>[4x]AMAISDPQAENPIFTDVFTADPAALVHKGRVYLYAGRDEAPDNTTFFVMNEWLVYSSDDMANWEAHGPGLRAKDFTWAKGDAWASQVIERNGKFYWYVTVRHDDTKPGFAIGVAVGDSPIGPFKDALGKALITNDMTTD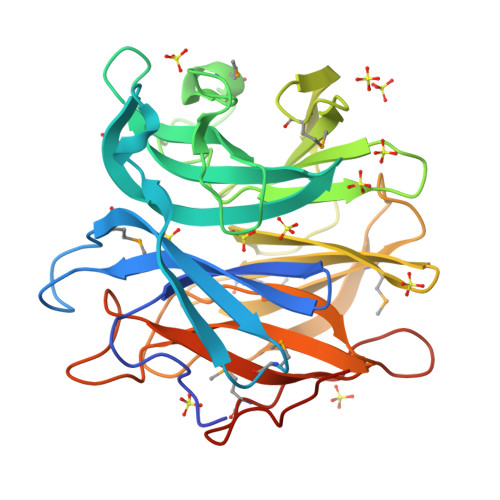TPIDWDDIDPSVFIDDDGQAYLFWGNTRPRYAKLKKNMVELDGPIRAIEGLPEFTEAIWVHKYQDNYYLSYAMGFPEKIGYAMGKSIKGPWVYKGILNEVAGNTPTNHQAIIEFNNKHYFIYHTGAGRPDGGQYRRSVSIDELFYNPDGTIKRIVMTTEGVAPNKSPERVKKAAK>[4x]VPVPVPVAVSGATTAGLRAQAARLAGHLRERPALGPEAVARPLLLSRAQRERRAV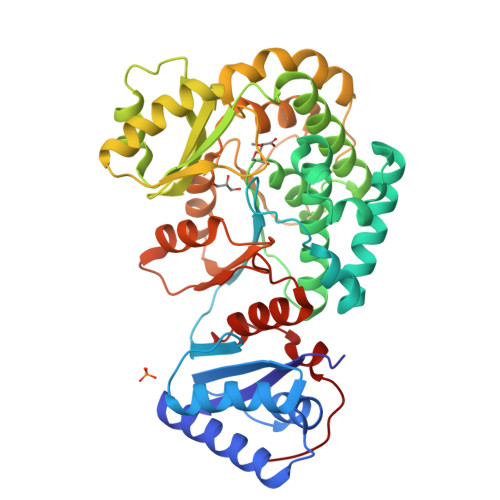VVAADRDSLLTGLDALAGGEAGPRLASGAADVTGRVVLVFPGQGAHWTGVAERLWREAPVFADSMARCADVLRDLAGWELREVLVDPVALERVDVLQPVSFAVVVSLAALWASVGVRPDAVVGHSQGEVAAAHVAGALTLAEAARIVVLRSALIARELSGRGAMLTVVADVERVTALLAGFEGRVCVAAVNGPASVTVSGEDGAVREFERVLSARRMLRWRLPGVDFAGHSPQVDALRAELLAALGDIASREPEIPLLSTVTGEPATRLDAEHWYRNLREPVRFADAVTALLDRGHRVFVEVSPHPVLTTSVVDLAAPHRTAVVGTLRRDEGGLDRFLLSAAELHVRGVPVDLARHAGAGTAEVP> QEPTDTPVSHDDTIVVTAAEQNLQAPGVSTITADEIRKNPVARDVSKIIRTMPGVNLTGNSTSGQRGNNRQIDIRGMGPENTLILIDGKPVSSRNSVRQGWRGERDTRGDTSWVPPEMIERIEVLRGPAAARYGNGAAGGVVNIITKKGSGEWHGSWDAYFNAPEHKEEGATKRTNFSLTGPLGDEFSFRLYGNLDKTQADAWDINQGHQSARAGTYATTLPAGREGVINKDINGVVRWDFAPLQSLELEAGYSRQGNLYAGDTQNTNSDSYTRSKYGDETNRLYRQNYALTWNGGWDNGVTTSNWVQYEHTRNSRIPEGLAGGTEGKFNEKATQDFVDIDLDDVMLHSEVNLPIDFLVNQTLTLGTEWNQQRMKDLSSNTQALTGTNTGGAIDGVSTTDRSPYSKAEIFSLFAENNMELTDSTIVTPGLRFDHHSIVGNNWSPALNISQGLGDDFTLKMGIARAYKAPSLYQTNPNYILYSKGQGCYASAGGCYLQGNDDLKAETSINKEIGLEFKRDGWLAGVTWFRNDYRNKIEAGYVAVGQNAVGTDLYQWDNVPKAVVEGLEGSLNVPVSETVMWTNNITYMLKSENKTTGDRLSIIPEYTLNSTLSWQAREDLSMQTTFTWYGKQQPKKYNYKGQPAVGPETKEISPYSIVGLSATWDVTKNV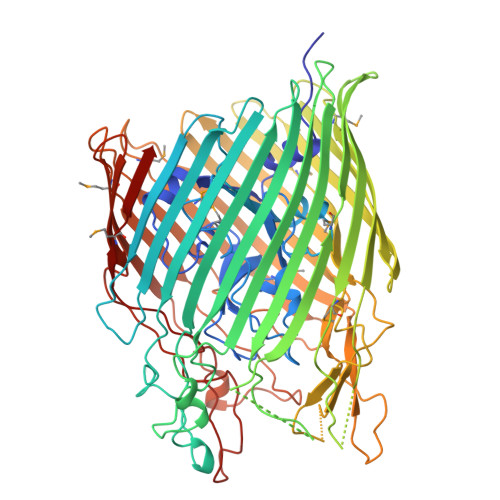SLTGGVDNLFDKRLWRAGNAQTTGDLAGANYIAGAGAYTYNEPGRTWYMSVNTHF> QVAYLNSLITDPNATKHVLYIHMGEPKTNNWDRELYVNPTTELQSGKTYTLKLRVKTSAACDVT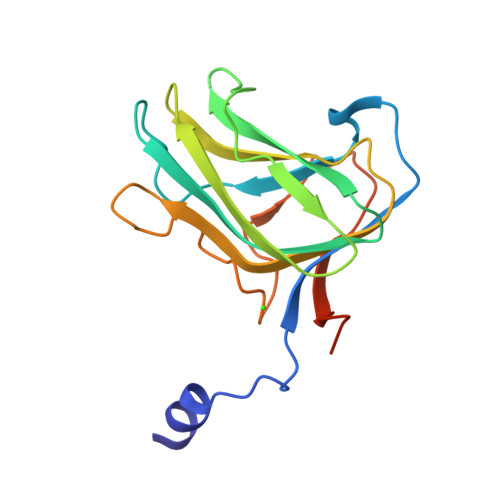VWPQGDATQYWPTPSFKSTTEWTTVAQAFEAKSALKQLRFELGTLGGDIWMDDVQLLDPDGNNLIANGTFEENADGWTKPSWHEYEIKTVADPDQEGGGGGMTE> VLSGALCFRMKDSALKV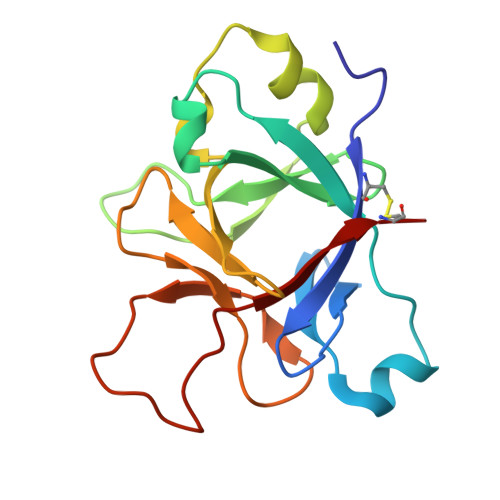LYLHNNQLLAGGLHAEKVIKGEEISVVPNRALDASLSPVILGVQGGSQCLSCGTEKGPILKLEPVNIMELYLGAKESKSFTFYRRDMGLTSSFESAAYPGWFLCTSPEADQPVRLTQIPEDPAWDAPITDFYFQQCD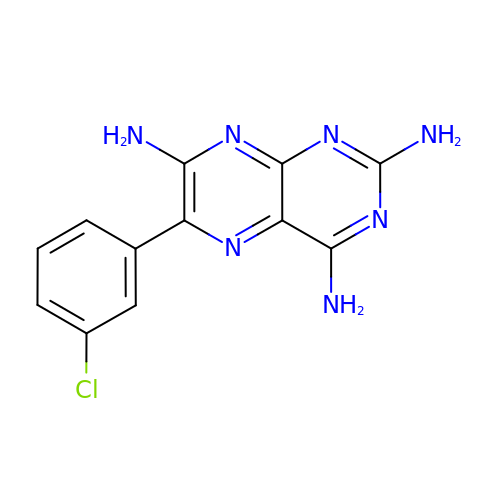6-(3-chlorophenyl)pteridine-2,4,7-triamine | C12 H10 Cl N7 | ZWNKKZSRANLVEW-UHFFFAOYSA-N>GGSRRILLPKNVIVECMVATHHNS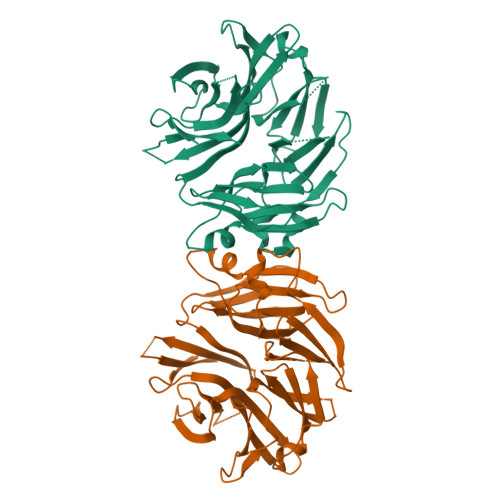RNASIWLGCGHTDRGQLSFLDLNTEGYTSEEVADSRILCLALVHLPVEKESWIVSGTQSGTLLVINTEDGKKRHTLEKMTDSVTCLYCNSFSKQSKQKNFLLVGTADGKLAIFEDKTVKLKGAAPLKILNIGNVSTPLMCLSESTNSTERNVMWGGCGTKIFSFSNDFTIQKLIETRTSQLFSYAAFSDSNIITVVVDTALYIAKQNSPVVEVWDKKTEKLCGLIDCVHFLREVMVKENKESKHKMSYSGRVKTLCLQKNTALWIGTGGGHILLLDLSTRRLIRVIYNFCNSVRVMMTAQLGSLKNVMLVLGYNRKNTEGTQKQKEIQSCLTVWDINLPHEVQNLEKHIEVRKELAEKMRRTSVE[2x]>MFIQEPKKLIDTGEIGNASTGDILFDGGNKINSDFNAIYNAFGDQRKMAVANGTGADGQIIHATGYYQKHSITEYATPVKVGTRHDIDTSTVGVKVIIERGELGDCVEFINSNGSISVTNPLTIQAIDSIKGVSGNLVVTSPYSKVTLRCISSDNSTSVWNYSIE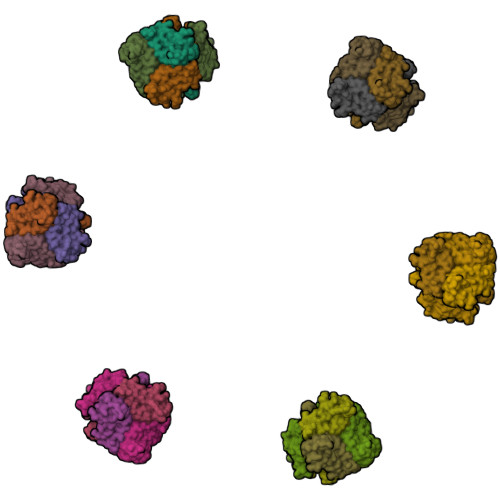SMFGQKESPAEGTWNISTSGSVDIPLFHRTEYNMAKLLVTCQSVDGRKIKTAEINILVDTVNSEVISSEYAVMRVGNETEEDEIANIAFSIKENYVTATISSSTVGMRAAVKVIATQKIGVAQ[18x]> M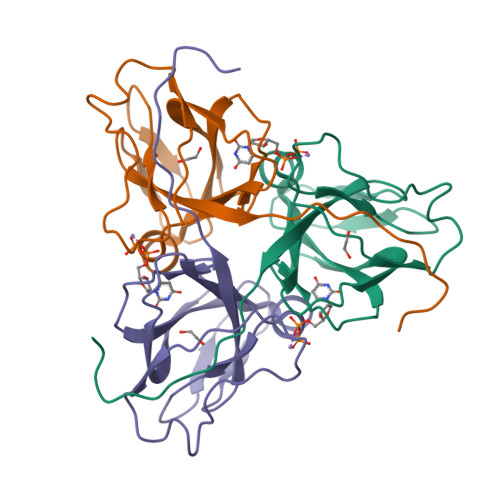MKKIDVKILDPRVGKEFPLPTYATSGSAGLDLRACLNDAVELAPGDTTLVPTGLAIHIADPSLAAMMLPRSGLGHKHGIVLGNLVGLIDSDYQGQLMISVWNRGQDSFTIQPGERIAQMIFVPVVQAEFNLVEDFDATDRGEGGFGHSGRQ>[3x]MTYETILVERDQRVGIITLNRPQALNALNSQVMNEVTSAATELDDDPDIGAIIITGSAKAFAAGADIKEMADLTFADAFTADFFATWGKLAAVRTPTIAAVAGYALGGGCELAMMCDVLIAADTAKFGQPEIKLGVLPGMGGSQRLTRAIGKAKAMDLILTGRTMDAAEAERSGLVSRVVPADDLLTEARATATTISQMSASAARMAKEAVNRAFESSLSEGLLYER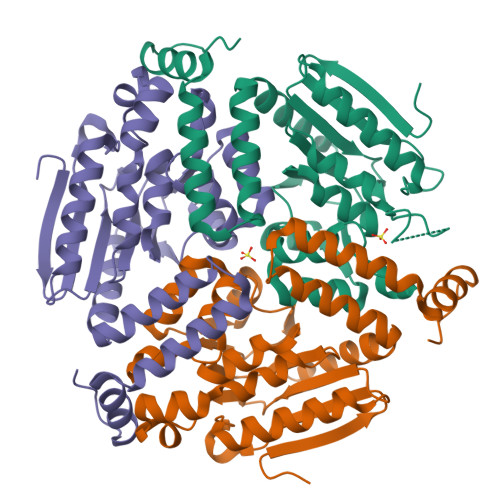RLFHSAFATEDQSEGMAAFIEKRAPQFTHR(5~{R},6~{R},7~{S},8~{S})-5-(hydroxymethyl)-2-(3-phenylpropyl)-5,6,7,8-tetrahydroimidazo[1,2-a]pyridine-6,7,8-triol | C17 H22 N2 O4 | 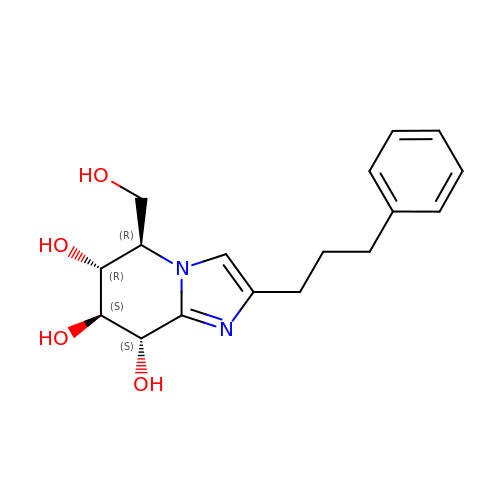QMUUATILFYBNFB-LVQVYYBASA-N>GSHMFNMLEQQIIHSQDMAHFRSEFFYVNHEHRENYEALLIYYKNSIDNPIVDGACY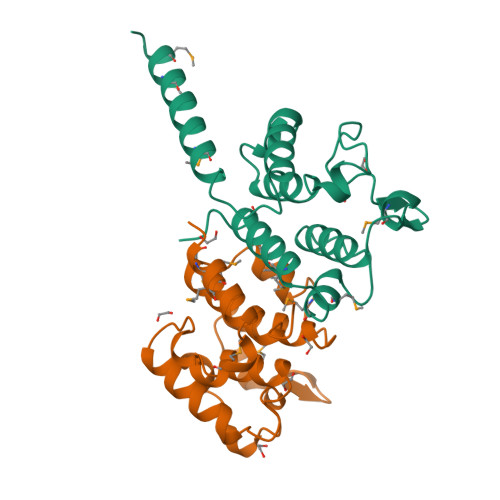ILALPEIFNSVDVFESELPFSWVYDENGITETMKSLSIPLQYLVAAALEVTDVNIFKPSGFTMGMNNWNIAQMRIFWQYTAIIRKEAL[2x]> ADNLAEFHVQNQECDSCHTPDGELSNDSLTYENTQCVSCHGTLAEVAETTKHEHYNAHASHFPGEVACTSCHSAHEKSMVYCDSCHSFDFNMPYAKKWLRDEPTIAELAKDKSERQAALASAPHDTVDVVVVGSGGAGFSAAISATDSGAKVILIEKEPVIGGNAKLAAGGMNAAWTDQQKAKKITDSPE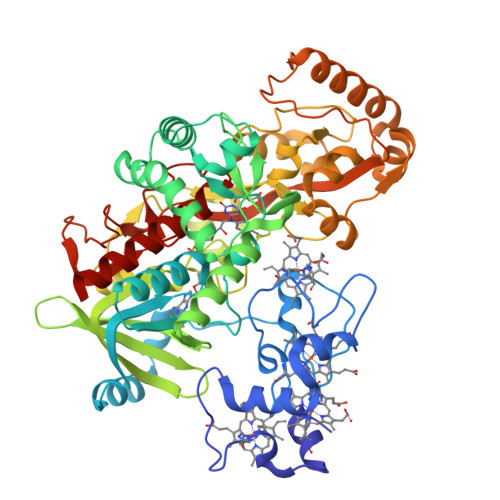LMFEDTMKGGQNINDPALVKVLSSHSKDSVDWMTAMGADLTDVGMMGGASVNRAHRPTGGAGVGAHVVQVLYDNAVKRNIDLRMNTRGIEVLKDDKGTVKGILVKGMYKGYYWVKADAVILATGGFAKNNERVAKLDPSLKGFISTNQPGAVGDGLDVAENAGGALKDMQYIQAHPTLSVKGGVMVTEAVRGNGAILVNREGKRFVNEITTRDKASAAILAQTGKSAYLIFDDSVRKSLSKIDKYIGLGVAPTADSLVKLGKMEGIDGKALTETVARYNSLVSSGKDTDFERPNLPRALNEGNYYAIEVTPGVHATMGGVMIDTKAEVMNAKKQVIPGLYGAGEVTGGVHGANRLGGNAISDIITFGRLAGEEAAKYSKKN> MQRSPLEKASVVSKLFFSWTRPILRKGYRQRLELSDIYQIPSVDSADNLSEKLEREWDRELASKKNPKLINALRRCFFWRFMFYGIFLYLGEVTKAVQPLLLGRIIASYDPDNKEERSIAIYLGIGLCLLFIVRTLLLHPAIFGLHHIGMQMRIAMFSLIYKKTLKLSSRVLDKISIGQLVSLLSNNLNKFDEGLALAHFVWIAPLQVALLMGLIWELLQASAFCGLGFLIVLALFQAGLGRMMMKYRDQRAGKISERLVITSEMIENIQSVKAYCWEEAMEKMIENLRQTELKLTRKAAYVRYFNSSAFFFSGFFVVFLSVLPYALIKGIILRKIFTTISFCIVLRMAVTRQFPWAVQTWYDSLGAINKIQDFLQKQEYKTLEYNLTTTEVVMENVTAFWEEGFGELFEKAKQNNNNRKTSNGDDSLFFSNFSLLGTPVLKDINFKIERGQLLAVAGSTGAGKTSLLMVIMGELEPSEGKIKHSGRISFCSQFSWIMPGTIKENIIGVSYDEYRYRSVIKACQLEEDISKFAEKDNIVLGEGGITLSGGQRARISLARAVYKDADLYLLDSPFGYLDVLTEKEIFESCVCKLMANKTRILVTSKMEHLKKADKILILHEGSSYFYGTFSELQNLQPDFSSKLMGCDSFDQFSAERRNSILTETLHRFSLEGDAPVSWTETKKQSFKQTGEFGEKRKNSILNPINSIRKFSIVQKTPLQMNGIEEDSDEPLERRLSLVPDSEQGEAILPRISVISTGPTLQARRRQSVLNLMTHSVNQGQNIHRKTTASTRKVSLAPQANLTELDIYSRRLSQETGLEISEEINEEDLKECFFDDMESIPAVTTWNTYLRYITVHKSLIFVLIWCLVIFLAEVAASLVVLWLLGNTPLQDKGNSTHSRNNSYAVIITSTSSYYVFYIYVGVADTLLAMGFFRGLPLVHTLITVSKILHHKMLHSVLQAPMSTLNTLKAGGILNRFSKDIAILDDLLPLTIFDFIQLLLIVIGAIAVVAVLQPYIFVATVPVIVAFIMLRAYFLQTSQQLKQLESEGRSPIFTHLVTSLKGLWTLRAFGRQPYFETLFHKALNLHTANWFLYLSTLRWFQMRIEMIFVIFFIAVTFISILTTGEGEGRVGIILTLAMNIMSTLQWAVNSSIDVDSLMRSVSRVFKFIDMPTEGKPTKSTKPYKNGQLSKVMIIENSHVKKDDIWPSGGQMTVKDLTAKYTEGGNAILENISFSISPGQRVGLLGRTGSGKSTLLSAFLRLLNTEGEIQIDGVSWDSITLQQWRKAFGVIPQKVFIFSGTFRKNLDPYEQWSDQEIWKVADEVGLRSVIEQFPGKLDFVLVDGGCVLSHGHKQLMCLARSVLSKAKILLLDQPSAHLDPVTYQIIRRTLKQAFADCTVILCEHRIEAMLECQQFLVIEENKVRQYDSIQKLLNERSLFRQAISPSDRVKLFPHRNSSKCKSKPQIAALKEETEEEVQDTRL

CFTR belongs to the ATP-binding cassette (ABC) transporter family but functions as an ATP-gated anion channel. It contains an N-terminal interfacial structure called the lasso motif, two transmembrane domains (TMDs) that form an anion conduction pathway, two cytoplasmic nucleotide-binding domains (NBDs) that bind and hydrolyze ATP, and a unique regulatory (R) domain that must be phosphorylated to open the channel. The predominant mutation causing cystic fibrosis, the deletion of phenylalanine 508 (Δ508) in the cystic fibrosis transmembrane conductance regulator (CFTR), leads to severe defects in CFTR biogenesis and function. The structure of wild type (WT) CFTR shows that F508 resides on the surface of NBD1, where it makes extensive interactions with the cytosolic region of TM helix 11 and intracellular loop 4 (8, 17).

In contrast, the type III corrector elexacaftor (VX-445) stabilized NBD1, resulting in a cryo-EM reconstruction of 3.7 Å resolution with ordered NBDs. The TMDs of elexacaftor-bound Δ508 CFTR closely resemble those of full-length CFTR in the phosphorylated, ATP-bound conformation, but the NBDs are very different. Elexacaftor-bound Δ508 has a “cracked-open” NBD dimer in which the catalysis-incompetent (degenerate) site is solvent accessible, and ATP makes contacts exclusively with the NBD1 face of the composite site. Elexacaftor partially, when used alone, and fully, when combined with a type I corrector, rectified interdomain assembly defects in Δ508 CFTR. In contrast, the binding site for elexacaftor (VX-445) has not previously been observed. The binding pocket is much shallower than that of type I correctors, as if the drug molecule is patched onto the surface of CFTR. The dual-function modulator elexacaftor (VX-445) engages TM helices 10-11 and the lasso motif, all of which are important for CFTR folding and function. Although the details of how elexacaftor potentiates CFTR await incisive electrophysiology measurements, our structural observations indicate that elexacaftor stabilizes TM 10-11, thereby strengthens the TMD/NBD1 interface, which is particularly vulnerable to disease-causing mutations.N-ACETYL GLUCONOLACTAM | C8 H14 N2 O5 | 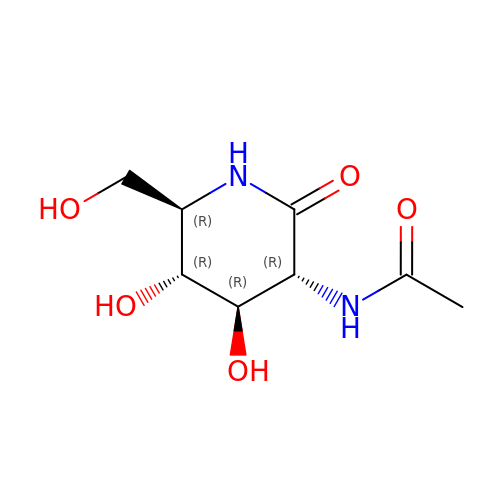DLGBPZFGIMUEIM-DBRKOABJSA-N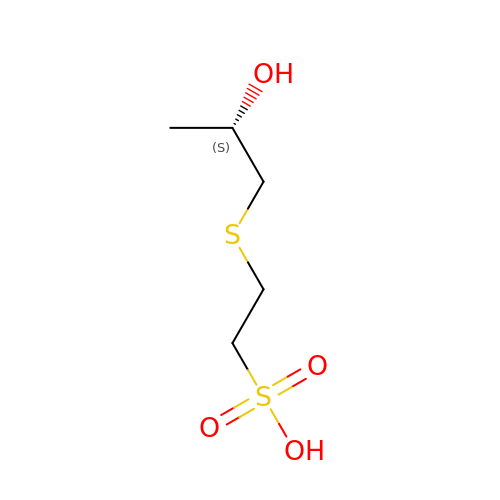2-{[(2S)-2-hydroxypropyl]sulfanyl}ethanesulfonic acid | C5 H12 O4 S2 | QWNJCCLFGYAGRK-YFKPBYRVSA-N> MDSTSTIANKIEEYLGAKSDDSKIDELLKADPSEVEYYRSGGDGDYLKNNICKITVNHSDSGKYDPCEKKLPPYDDNDQWKCQQNSSDGSGKPENICVPPRRERLCTYNLENLKFDKIRDNNAFLADVLLTARNEGEKIVQNHPDTNSSNVCNALERSFADLADIIRGTDQWKGTNSNLEKNLKQMFAKIRENDKVLQDKYPKDQKYTKLREAWWNANRQKVWEVITCGARSNDLLIKRGWRTSGKSDRKKNFELCRKCGHYEKEVPTKLDYVPQFLRWLTEWIEDFYREKQNLIDDMERHREECTREDHKSKEGTSYCSTCKDKCKKYCECVKKWKTEWENQENKYKDLYEQNKNKTSQKNTSRYDDYVKDFFEKLEANYSSLENYIKGDPYFAEYATKLSFILNPSDANNPSGETANHNDEACNCNESGISSVGQAQTSGPSSNKTCITHSSIKTNKKKECKDVKLGVRENDKDLKICVIEDTSLSGVDNCCCQDLLGILQENCSDNKRGSSSNDSCDNKNQDECQKKLEKVFASLTNGYKCDKCKSGTSRSKKKWIWKKSSGNEEGLQEEYANTIGLPPRTQSLYLGNLPKLENVCEDVKDINFDTKEKFLAGCLIVSFHEGKNLKKRYPQNKNSGNKENLCKALEYSFADYGDLIKGTSIWDNEYTKDLELNLQNNFGKLFGKYIKKNNTAEQDTSYSSLDELRESWWNTNKKYIWTAMKHGAEMNITTCNADGSVTG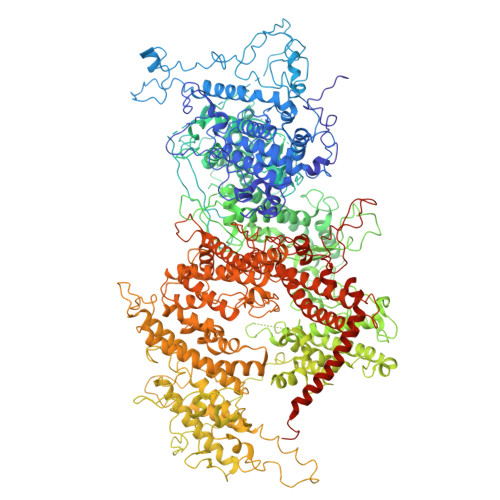SGSSCDDIPTIDLIPQYLRFLQEWVENFCEQRQAKVKDVITNCKSCKESGNKCKTECKTKCKDECEKYKKFIEACGTAGGGIGTAGSPWSKRWDQIYKRYSKHIEDAKRNRKAGTKNCGTSSTTNAAASTDENKCVQSDIDSFFKHLIDIGLTTPSSYLSNVLDDNICGADKAPWTTYTTYTTTEKCNKERDKSKSQSSDTLVVVNVPSPLGNTPYRYKYACQCKIPTNEETCDDRKEYMNQWSCGSARTMKRGYKNDNYELCKYNGVDVKPTTVRSNSSKLDGNDVTFFNLFEQWNKEIQYQIEQYMTNANISCIDEKEVLDSVSDEGTPKVRGGYEDGRNNNTDQGTNCKEKCKCYKLWIEKINDQWGKQKDNYNKFRSKQIYDANKGSQNKKVVSLSNFLFFSCWEEYIQKYFNGDWSKIKNIGSDTFEFLIKKCGNNSAHGEEIFSEKLKNAEKKCKENESTDTNINKSETSCDLNATNYIRGCQSKTYDGKIFPGKGGEKQWICKDTIIHGDTNGACIPPRTQNLCVGELWDKSYGGRSNIKNDTKELLKEKIKNAIHKETELLYEYHDTGTAIISKNDKKGQKGKNDPNGLPKGFCHAVQRSFIDYKNMILGTSVNIYEHIGKLQEDIKKIIEKGTPQQKDKIGGVGSSTENVNAWWKGIEREMWDAVRCAITKINKKNNNSIFNGDECGVSPPTGNDEDQSVSWFKEWGEQFCIERLRYEQNIREACTINGKNEKKCINSKSGQGDKIQGACKRKCEKYKKYISEKKQEWDKQKTKYENKYVGKSASDLLKENYPECISANFDFIFNDNIEYKTYYPYGDYSSICSCEQVKYYKYNNAEKKNNKSLCYEKDNDMTWSKKYIKKLENGRSLEGVYVPPRRQQLCLYELFPIIIKNEEGMEKAKEELLETLQIVAEREAYYLWKQYNPTGKGIDDANKKACCAIRGSFYDLEDIIKGNDLVHDEYTKYIDSKLNEIFGSSNTNDIDTKRARTDWWENETITNGTDRKTIRQLVWDAMQSGVRYAVEEKNENFPLCMGVEHIGIAKPQFIRWLEEWTNEFCEKYTKYFEDMKSKCDPPKRADTCGDNSNIECKKACANYTNWLNPKRIEWNGMSNYYNKIYRKSNKESEDGKDYSMIMAPTVIDYLNKRCHGEINGNYICCSCKNIGAYNTTSGTVNKKLQKKETECEEEKGPLDLMNEVLNKMDKKYSAHKMKCTEVYLEHVEEQLNEIDNAIKDYKLYPLDRCFDDQTKMKVCDLIADAIGCKDKTKLDELDEWNDMDLRGTYNKHKGVLIP>[3x]SQQLQKEEEARKVKSGIRQMRLFSQDECAKIEARIDEVVSRAEKGLY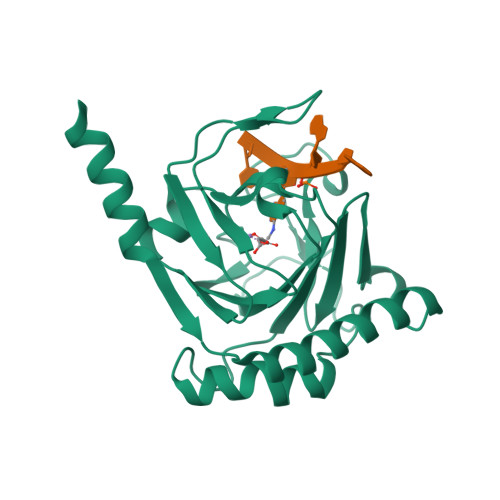NEHTVDRAPLRNKYFFGEGYTYGAQLQKRGPGQERLYPPGDVDEIPEWVHQLVIQKLVEHRVIPEGFVNSAVINDYQPGGCIVSHVDPIHIFERPIVSVSFFSDSALCFGCKFQFKPIRVSEPVLSLPVRRGSVTVLSGYAADEITHCIRPQDIKERRAVIILRKTRLDAPRL>RSPWDPPVPKHISPYTPRTRIAIEVEKAFDDCMRQNWCSVNNPYLAKSVSLLSFLSLNHPTEFIKVLPLIDFDPLVTFYLLLEPYKTHGDDFLIPETILFGPTGWNGTDLYQSAMLEFKKFFTQITRQTFMDIADSATKEVDVPICYSDPETVHSYTNHVRTEILHHNAVNKVTTPNLVVQAYNELEQTNTIRHYGPIFPESTINALRFWKKLWQDEQRFVIHGLHRTLMDQPTYETSEFAEIVRNLRFSRPGNNYINELNITSPAMYGDKHTTGDIAPNDRFAMLVAFINSTDFLYTAIPEEKVGGNLESRGPFEGKPIPNPLLGLDSTRTGHHHHH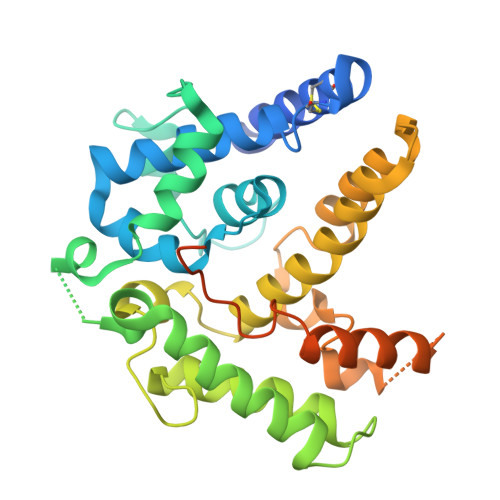H[2x]>MVKVGINGFGRIGRLVMRASLEHPEVQVVAVNDPFIDLEYMEYMFKYDSTHGRFKGTTEVKDGKLVINGNPISVYALKDPAAIPWKEAGADFVVESTGVFTTTEKASAHLHGGAKKVIISAPSADAPMFVMGVNEKTYDAATMNVVSNASCTTNCLAPLAKVINDNFGIEEGLMTTIHAYTATQKTVDGPSGKKWRDGRGANQNVIPATTGAAKAVGKVIPELNGKLTGMAFRVPVPDVSVVDLTCRLKKPTSYEEIKKVVKKASETDLKGFLAYTEDQVVSSDFISDTHSSVFDALAGIQLNPTFVKLVSWYDNEYGYSHRVVDLIEYMATKAENLYFQSHH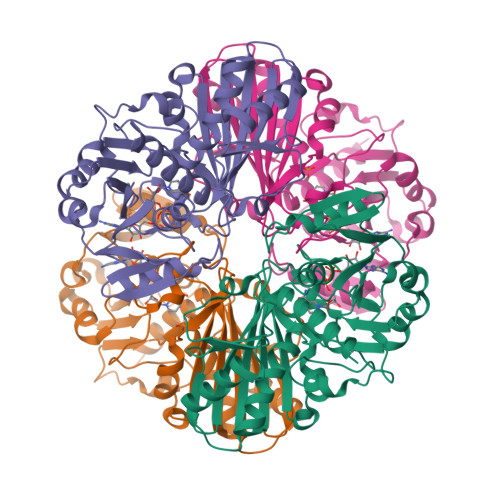HHHHDYKDDDDK[8x]3-[(1-Carboxyvinyl)oxy]benzoic acid | C10 H8 O5 | 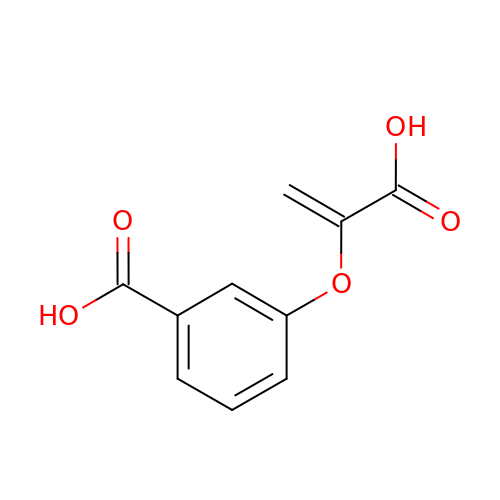HGVAHYJMDVROLE-UHFFFAOYSA-N> MRWISGLDLVAHQMTARKKNSMALNEADTCRVYVTPKLKESGWENNPSAITEQYTFTDGRVQFKGSKVQRGEQKRADYLLKYTRDFPIAVVEAKPENSPVGQGMQQAKDYAEILGLKFAYSTNGHEILEFDYTTGEEQLLSRFPTPDELFKRLCGDEGIKDEDLDTLLSPYHHVSGYSPRYYQQIAINRAVQSVLQGKKRSLITMATGTGKTVVAFQISWKLWSARWNRTGDYRKPRILFLADRNVLVDDPKDKTFTPFGDARHKIEGGKVVKSREIYFAIYQSIASDERRPGLYKEFPQDFFDLIIIDECHRGSARDNSNWREILEYFEPAFQIGMTATPLREDNRDTYRYFGNPIYTYSLRQGIDDGFLAPYRVHRVISEVDAAGWRPSKGDVDRFGREIPDGEYQTKDFERVIALKART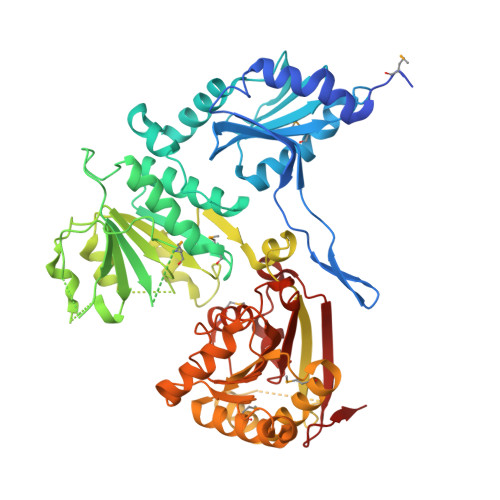DAFAKHLTDFMKRTDRFAKTIVFCVDQEHADEMRRALNNLNSDLSRKHPDYVARVTSEEGKIGKGHLSRFQELETSTPVILTTSQLLTTGVDAPTCKNVVLARVVNSMSEFKQIVGRGTRLREDYGKLWFNIIDYTGSATQNFADPDFDGYPEIEDEVVIDEDGEEVV>[2x]GPDSMPRGADQENMLKISGYPGMLNTFGIAQLLTPYRVNGITITGAQSAVVALENKFQVYQAVQDFNGKKLDRNHKLQVSSLVV;>GPDSMASSS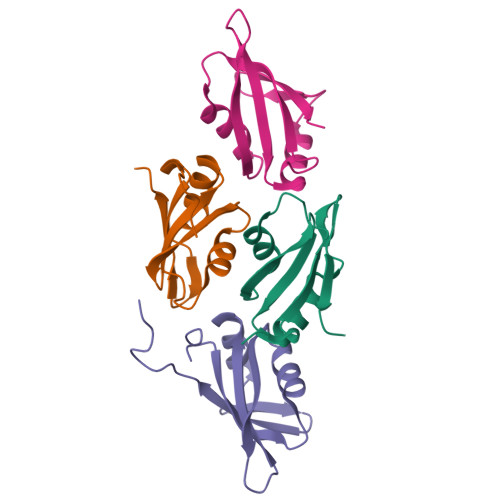TAYYLKDAGFHIRNIPKAWNDWNLFHVFQNFGKVSYCRVVGQSNDGQVQLGFVNMMSVADADEVRKNLNDGNLIGENFTLKVTDHKNVGGSLLP[2x]> MRGSHHHHHHTDPQGDAAQKTDTSHHDQDHPTFNKITPNLAEFAFSLYRQLAHQSNSTNIFFSPVSIATAFAMLSLGTKADTHDEILEGLNFNLTEIPEAQIHEGFQELLRTLNQPDSQLQLTTGNGLFLSEGLKLVDKFLEDVKKLYHSEAFT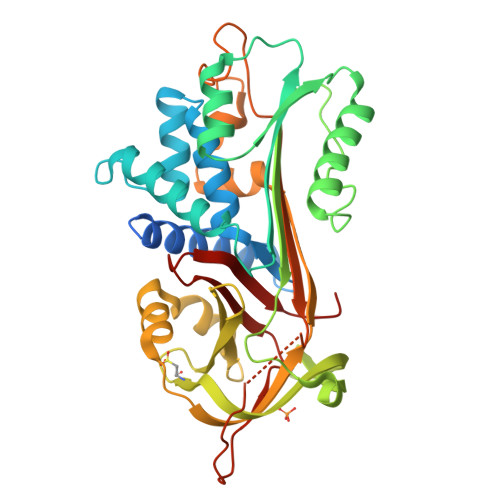VNFGDTEEAKKQINDYVEKGTQGKIVDLVKELDRDTVFALVNYIFFKGKWERPFEVKDTEEEDFHVDQVTTVKVPMMKRLGMFNIQHCKKLSSWVLLMKFLGNATAIFFLPDEGKLQHLENELTHDIITKFLENEDRRSASLHLPKLSITGTYDLKSVLGQLGITKVFSNGADLSGVTEEAPLKLSKAVHKAVLTIDEKGTEAAGAMFLEAIPMSIPPEVKFNKPFVFLMIEQNTKSPLFMGKVVNPTQK> SCELYHYQECVRGTTVILKEPCPSGTYEGNSPFHPLADNKFALTCTSTHFAFACADGTRHTYQLRARSVSPKLFIRQ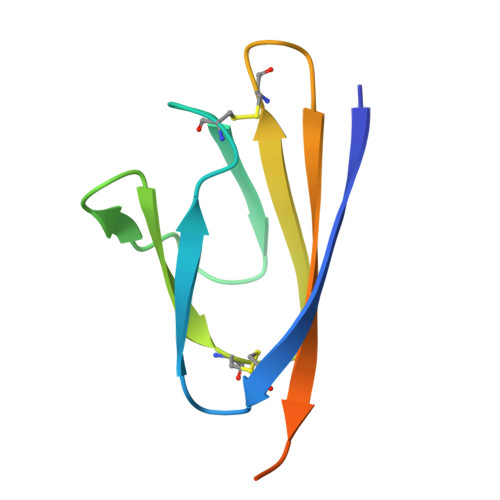EEVQQE4-[(1,1-dioxido-1,2-thiazetidin-2-yl)carbonyl]morpholine | C7 H12 N2 O4 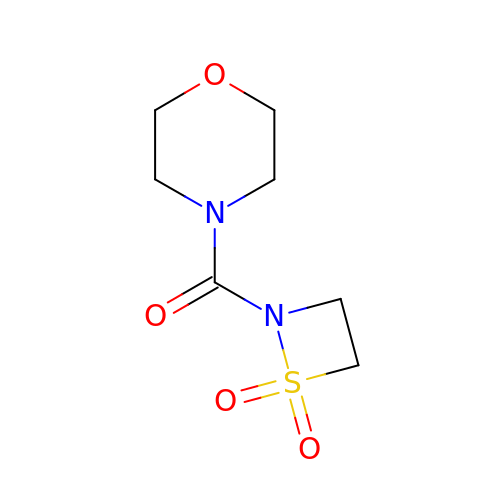S | FLIYHWNBIOGIBH-UHFFFAOYSA-N>GMERGIV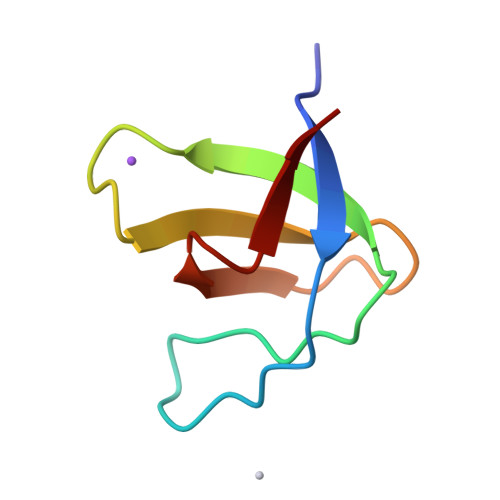QYDFMAESQDELTIKSGDKVYILDDKKSKDWWMCQLVDSGKSGLVPAQFIEPV[2x]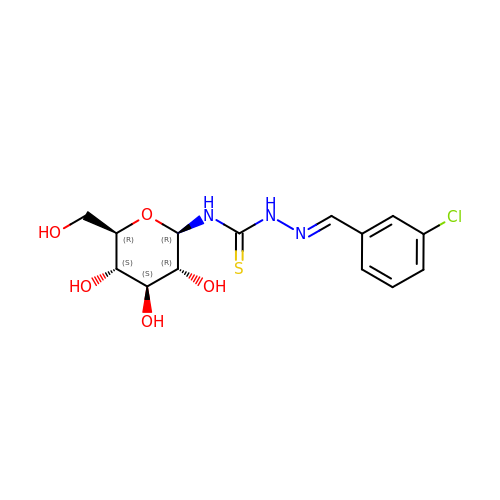N-({(2E)-2-[(3-chlorophenyl)methylidene]hydrazino}carbonothioyl)-beta-D-glucopyranosylamine | C14 H18 Cl N3 O5 S | ADXZJKYCOSNBPM-QCOQDYPWSA-N5-methyl-6-{[4-(trifluoromethoxy)phenyl]sulfanyl}thieno[2,3-d]pyrimidine-2,4-diamine | C14 H11 F3 N4 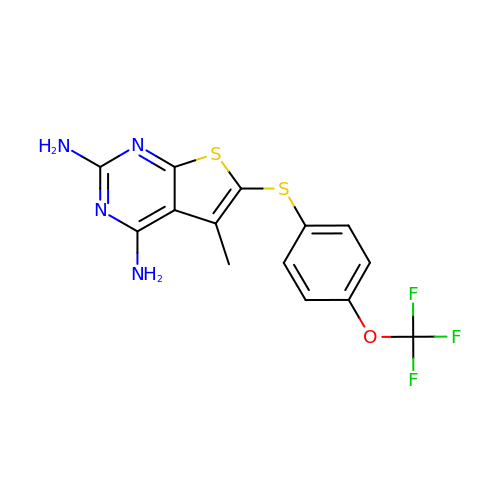O S2 | HDFJEMJYJKUGRK-UHFFFAOYSA-N>ENNVTKVKDTNIFPYTGVVAFKSATGFVVGKNTILTNKHVSKNYKVGDRITAHPNSDKGNGGIYSIKKIINYPGKEDVSVIQVEERAIERGPKGFNFNDNVTPFKYAAGAKAGERIKVIGYPHPYKNKYVLYESTGPVMSVEGSSIVYSAHTESGNSGSPVLNSNNELVGIHFASDVKNDDNRNAYGVYFTPEIKKFIA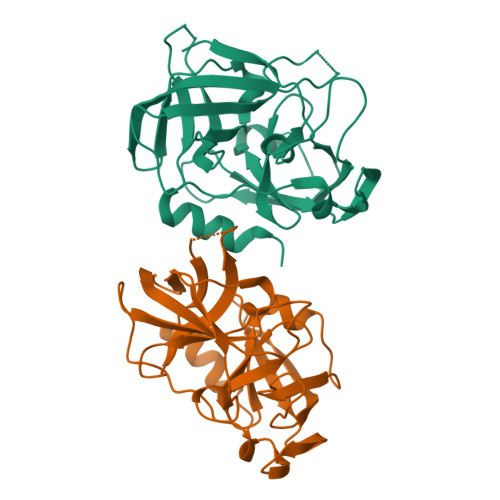ENIDK[2x]> SINNGTFDEPIVNDQANNPDEWFIWQAGDYGISGARVSDYGVRDGYAYITIADPGTDTWHIQFNQWIGLYRGKTYTISFKAKADTPRPINVKILQNHDPWTNYFAQTVNLTADWQTFTFTYTHPDDADEVVQI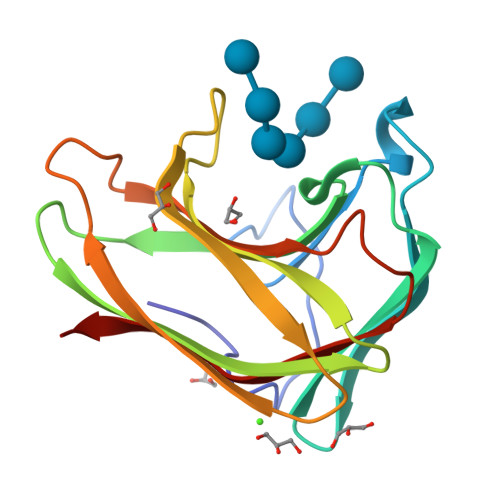SFELGEGTATTIYFDDVTVSPQ2-({(4R)-4-(2-chlorophenyl)-2-[(6-fluoro-1,3-benzoxazol-2-yl)amino]-6-methyl-1,4-dihydropyrimidine-5-carbonyl}amino)pyridine-4-carboxylic 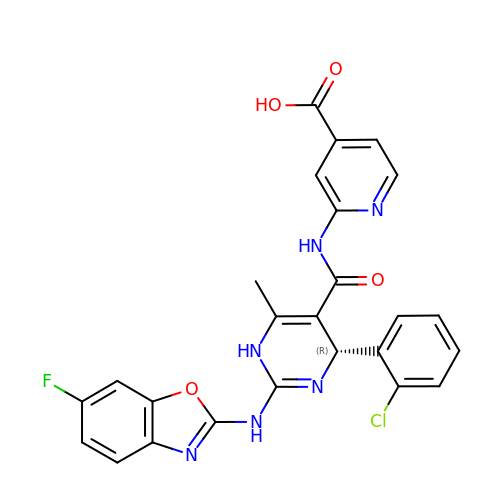acid | C25 H18 Cl F N6 O4 | MNTJOCWGZZCRNY-NRFANRHFSA-N In contrast, modification of cytoplasmic proteins with a single O-linked N-acetylglucosamine (O-GlcNAc)4 is a regulatory post-translational modification that is dependent on a single O-GlcNAc-transferase (OGT), which transfers the O-GlcNAc moiety onto target proteins, and O-GlcNAcase (OGA), which can reverse this process. In this report, we describe the identification of the first complete putative bacterial protein O-GlcNAcylation system, found in the soil thermophile Thermobaculum terrenum. We identified the products of genes Tter_2822 (hereafter Ttogt) and Tter_0116 (hereafter Ttoga) as putative OGT and OGA orthologues, respectively. To investigate the catalytic machinery and conservation of substrate/product binding modes, we determined the crystal structures of TtOGT and TtOGA.

Previous work has shown that mutation of the CpOGA catalytic acid Asp298 to asparagine (Asp120 in TtOGA) results in loss of activity, but the enzyme retains the ability to bind to substrates. TtOGA possessing an equivalent mutation (D120N) was utilized to trap a complex of TtOGA with a glycopeptide derived from the validated hTab1 glycosylation site (VPYgSSAQ). Synchrotron diffraction data were collected to 2.06 Å, and the structure was solved by molecular replacement. The TtOGA structure reveals a classic (β/α)8 barrel (TIM barrel) at the N terminus and a C-terminal helical bundle domain resembling those found in other bacterial OGA homologues. The TtOGA catalytic domain is similar to that of CpOGA and OgOGA (r.m.s.d. = 1.3 Å for 228 Cα atoms and 1.4 Å for 233 Cα atoms, respectively). In TtOGA, the active site residues involved in this mechanism are conserved: the catalytic acid (Asp120 in TtOGA) protonates the glycosidic bond, a neighboring aspartic acid (Asp119 in TtOGA) stabilizes the conformation of the 2-acetamido group, and the developing positive charge on the oxazolinium intermediate and an aspartic acid side chain (Asp228 in TtOGA) hydrogen bonds O4 and O6, stabilizing the formation of the transition state. The TtOGA C-terminal helical bundle domain, which has been proposed to play a role in recognition of the protein component of the substrates, comprises five helices (α11–α15) that are connected to the GH84 domain with two shorter helices (α9 and α10). However, in the absence of the α10-α11 loop, TtOGA recognizes the peptide component of the hTab1 glycopeptide by a sequence-independent hydrogen bond between Gly230 and the backbone carbonyl oxygen at the −3 subsite of the glycopeptide. Given the relatively better conservation between TtOGA and hOGA at the substrate binding groove, the TtOGA·hTab1-O-GlcNAc complex may provide an alternative or more accurate model to study hOGA-substrate interactions. The structural data further confirm the high level of structural conservation between TtOGA and CpOGA, and sequence alignments suggest that, in terms of loop structure and the peptide binding groove, TtOGA is a better structural model for hOGA.

>MEYFRYRGIIEGFYGKPWEHQERLDMFEFMQANNLNAYIYAPKQDLYHRELWREPYKEEQLQLFKELIEKAGSCGINFTFAISPGLSLVYSSEEELETLIRKITPFLEMGVHSIGIFFDNVPFDLIHEEDRNSYSNLAEAQADFLTRVLQRLESTISTPQIIMCPTFYCNDPNLEYLRILGQRLPKNIDVFWTGPNVCSHEITTSHMQEVQKSLQRPATLWDNYPVNDGGMMPELHIGPYDHRDPELHTHVVGIYANPMALPEASKLPLYTFAQYLNSPSQYNPQDSWRQAVSTLLGEDNLSAMEKFYQSNTISCLEPEEPAYLTNLFKKVQEDFASFRFEQGLRTLREEIISMQTTYSRLSTQDSKFFWEIRPWLEEYKLWTDYLDQAMITFSNLFTGFFTADEEQARESLQKALQGRTYLREVLKDAVDFRTRVCGDVVRNFLQQVLRSTVSIELQAEGKEWTALPPGIVRD[2x];>VPYSSAQ[2x]> MADHSASGAPALSTNIESGKFDEKAAEAAAYQPKPKVEDDEDEDIDALIEDLESHDGHDAEEEEEEATPGGGRVVPEDMLQTDTRVGLTSEEVVQRRRKYGLNQMKEEKENHFLKFLGFFVGPIQFVMEGAAVLAAGLEDWVDFGVICGLLLLNAVVGFVQEFQAGSIVDELKKTLALKAVVLRDGTLKEIEAPEVVPGDILQVEEGTIIPADGRIVTDDAFLQVDQSALTGESLAVDKHKGDQVFASSAVKRGEAFVVITATGDNTFVGRAAALVNAASGGSGHFTEVLNGIGTILLILVIFTLLIVWVSSFYRSNPIVQILEFTLAITIIGVPVGLPAVVTTTMAVGAAYLAKKKAIVQKLSAIESLAGVEILCSDKTGTLTKNKLSLHDPYTVAGVDPEDLMLTACLAASRKKKGIDAIDKAFLKSLKYYPRAKSVLSKYKVLQFHPFDPVSKKVVAVVESPQGERITCVKGAPLFVLKTVEEDHPIPEEVDQAYKNKVAEFATRGFRSLGVARKRGEGSWEILGIMPCMDPPRHDTYKTVCEAKTLGLSIKMLTGDAVGIARETSRQLGLGTNIYNAERLGLGGGGDMPGSEVYDFVEAADGFAEVFPQHKYNVVEILQQRGYLVAMTGDGVNDAPSLKKADTGIAVEGSSDAARSAADIVFLAPGLGAIIDALKTSRQIFHRMYAYVVYRIALSIHLEIFLGLWIAILNRSLNIELVVFIAIFADVATLAIAYDNAPYSQTPVKWNLPKLWGMSVLLGVVLAVGTWITVTTMYAQGENGGIVQNFGNMDEVLFLQISLTENWLIFITRANGPFWSSIPSWQLSGAIFLVDILATCFTIWGWFEHSDTSIVAVVRIWIFSFGIFCIMGGVYYILQDSVGFDNLMHGKSPKGNQKQRSLEDFVVSLQRVSTQHEKSQ

The plasma membrane of fungal and plant cells contains a proton-pumping P-type adenosine triphosphatase (ATPase) that maintains the intracellular pH and generates a proton-motive force, driving the import of nutrients by secondary transporters. Unlike any other known P-type ATPase, Pma1 is a hexamer that localizes to specific ordered microdomains in the fungal plasma membrane. Autoinhibited Pma1 hexamers in the plasma membrane of starving fungi are activated by glucose signaling and subsequent phosphorylation of the autoinhibitory domain. We have determined the structure of hexameric Pma1 from Neurospora crassa by electron cryo-microscopy at 3.3-Å resolution, elucidating the molecular basis for hexamer formation and autoinhibition and providing a basis for structure-based drug development.

An atomic model was built into the monomer map and then extended into a hexameric model by symmetry-assisted placement of five additional copies into the hexamer map. Our molecular model comprises >90% of all residues, lacking only the N-terminal extension (residues 1 to 65), and two loops (A-M3, residues 269 to 283, and M10-R, residues 881 to 891), for which no continuous density was visible in the map, probably because of flexibility. The domains of Pma1 are arranged in an E1 conformation, with the N domain in proximity to the P domain, as required for MgATP-mediated phosphorylation of Asp378. We added 600 μM AlFx to the sample before grid preparation, with the aim to stabilize the enzyme in its transition state of phosphorylation, E1~P. However, we did not find a clear density for AlFx in its expected position between the adenosine diphosphate (ADP) β-phosphate and the Asp378 carboxyl group. We have hence captured the basal state before ATP hydrolysis, occupied by excess MgADP. As expected for a prephosphorylation E1 state, access from the cytosol to the proton-binding site is open in our structure. The M1 helix with its characteristic 90° kink (induced by Pro123) is embedded deeply inside the membrane, forming a wide funnel-shaped access toward the H+ binding site in M6, similar to the Ca2+ entry funnel in SERCA (and see more detailed discussion below). The mouth of this access pathway is negatively charged because of the conserved Glu162 in M2, and it extends into a large aqueous cavity between M1, M2, M6, and an unwound region in M4 around the conserved Pro335. Asp730 is situated adjacent to the internal cavity and opposite the equally highly conserved Asn154 in M2, at a distance suitable for capturing a proton within a hydrogen bond (2.9 Å between the aspartate carboxyl and the asparagine amide). The additional C-terminal autoinhibitory R domain forms an α helix that folds against the P domain.> DERDRVQKKTFTKWVNKHLIKAQRHISDLYEDLRDGHNLIS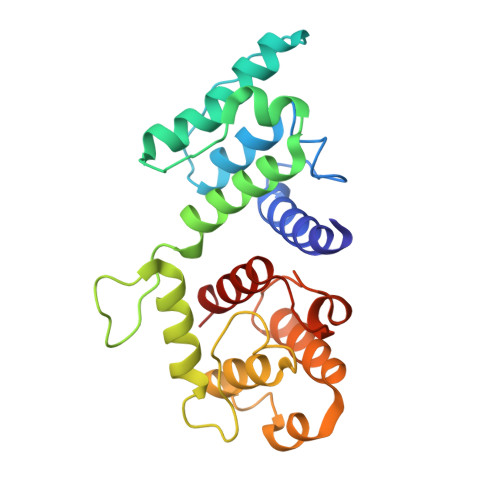LLEVLSGDSLPREKGRMRFHKLQNVQIALDYLRHRQVKLVNIRNDDIADGNPKLTLGLIWTIILHFQISDIQVSGQSEDMTAKEKLLLWSQRMVEGYQGLRCDNFTSSWRDGRLFNAIIHRHKPLLIDMNKVYRQTNLENLDQAFSVAERDLGVTRLLDPEDVDVPQPDEKSIITYVSSLYDAMP>GPLGSMEDAKNIKKGPAPFYPLEDGTAGEQLHKAMKRYALVPGTIAFTDAHIEVNITYAEYFEMSVRLAEAMKRYGLNTNHRIVVCSENSLQFFMPVLGALFIGVAVAPANDIYNERELLNSMNISQPTVVFVSKKGLQKILNVQKKLPIIQKIIIMDSKTDYQGFQSMYTFVTSHLPPGFNEYDFVPESFDRDKTIALIMNSSGSTGLPKGVALPHRNACVRFSHCRDPIFGNQIIPDTAILSVVPFHHGFGMFTTLGFLICGFRVVLMYRFEEELFLRTLQDYKIQSALLVPTLFSFFAKSTLIDKYDLSNLHEIASGGAPLSKEVGEAVAKRFNLPGIRQGYGLTETTSAILITPNGDDKPGAVGKVVPFFEAKVVDLDTGKTLGVNQRGELCVRGPMIMSGYVNNPEAT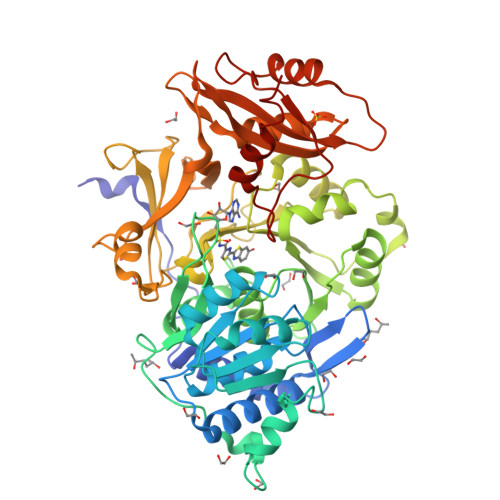NALIDKDGWLHSGDIAYWDEDEHFFIVDRLKSLIKYKGYQVAPAELESILLQHPNIFDAGVAGLPDDDAGELPAAVVVLEHGKTMTEKEIVDYVASQVTTAKKLRGGVVFVDEVPKGLTGKLDARKIREILIKAKKGGKSKL[3x]>IVGGHEAQPHSRPYMASLQMRGNPGSHFCGGTLIHPSFVLTAAHCLRDIPQRLVNVVLGAHNVRTQEPTQQHFSVAQVFLNNYDAENKLNDILLIQLSSPANLSASVATVQLPQQDQPVPHGTQCLAMGWGRVGAHDPPAQVLQELNVTVVTFFCRPHNICTFVPRRKAGICFGDSGGPLICDGIIQGIDSFVIWGCATR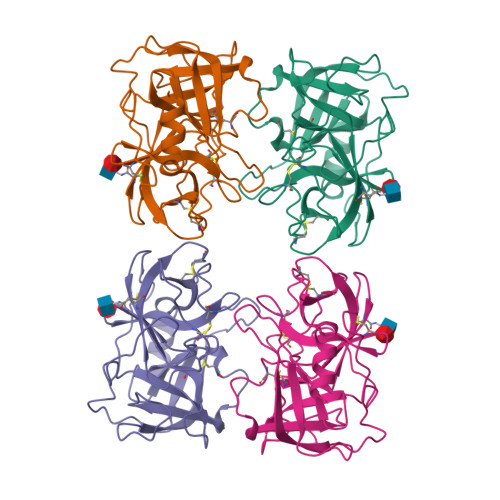LFPDFFTRVALYVDWIRSTLR[4x]> ISPIETVPVKLKPGMDGPKVKQWPLTEEKIKALVEICTEMEKEGKISKIGPENPYNTPVFAIKKKDSTKWRKLVDFRELNKRTQDFWEVQLGIPHPAGLEKKKSVTVLDVGDAYFSVPLDEDFRKYTAFTIPSINNETPGIRYQYNVLPQGWKGSPAIFQSSMTKILEPFRKQNPDIVIYQYMDDLYVGSDLEIGQHRTKIEELRQHLLRWGLTTPDKKHQKEPPFLWMGYELHPDKWTVQPIVLPEKDSWTVNDIQKLVGKLNWASQIY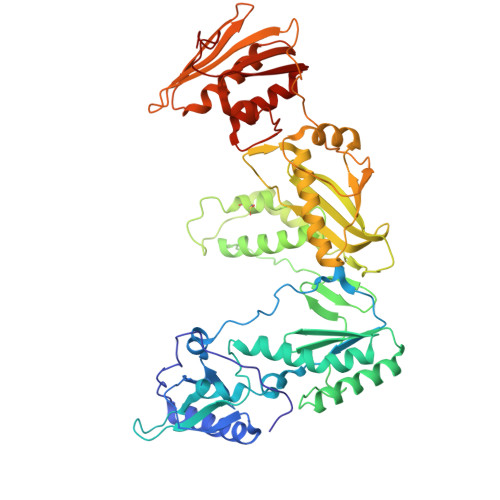PGIKVRQLCKLLRGTKALTEVIPLTEEAELELAENREILKEPVHGVYYDPSKDLIAEIQKQGQGQWTYQIYQEPFKNLKTGKYARMRGAHTNDVKQLTEAVQKITTESIVIWGKTPKFKLPIQKETWETWWTEYWQATWIPEWEFVNTPPLVKLWYQLEKEPIVGAETFYVDGAANRETKLGKAGYVTNRGRQKVVTLTDTTNQKTELQAIYLALQDSGLEVNIVTDSQYALGIIQAQPDQSESELVNQIIEQLIKKEKVYLAWVPAHKGIGGNEQV7-chloro-3-({4-hydroxy-1-[(3S)-3-phenylbutanoyl]piperidin-4-yl}methyl)quinazolin-4(3H)-one 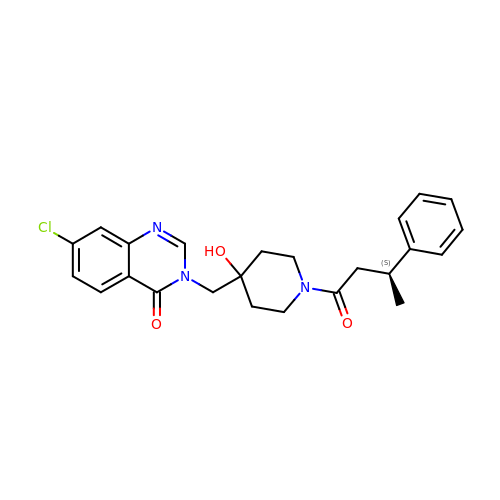| C24 H26 Cl N3 O3 | YRRYGKYWFQIDQT-KRWDZBQOSA-N>[2x]MVVTRIAPSPTGDPHVGTAYIALFNYAWARRNGGRFIVRIEDTDRARYVPGAEERILAALKWLGLSYDEGPDVAAPTGPYRQSERLPLYQKYAEELLKRGWAYRAFETPEELEQIRKEKGGYDGRARNIPPEEAEERARRGEPHVIRLKVPRPGTTEVKDELRGVVVYDNQEIPDVVLLKS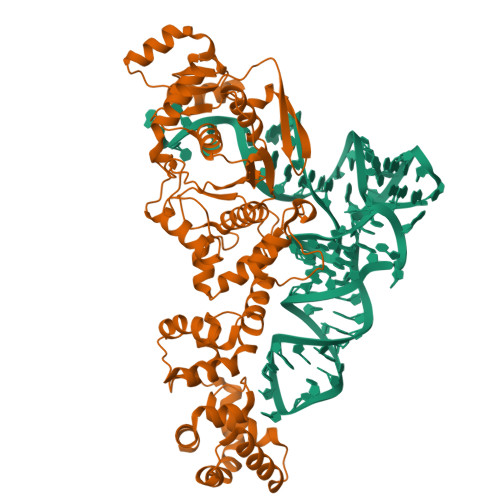DGYPTYHLANVVDDHLMGVTDVIRAEEWLVSTPIHVLLYRAFGWEAPRFYHMPLLRNPDKTKISKRKSHTSLDWYKAEGFLPEALRNYLCLMGFSMPDGREIFTLEEFIQAFTWERVSLGGPVFDLEKLRWMNGKYIREVLSLEEVAERVKPFLREAGLSWESEAYLRRAVELMRPRFDTLKEFPEKARYLFTEDYPVSEKAQRKLEEGLPLLKELYPRLRAQEEWTEAALEALLRGFAAEKGVKLGQVAQPLRAALTGSLETPGLFEILALLGKERALRRLERALA> PISPIETVPVKLKPGMDGPKVKQWPLTEEKIKALVEICTEMEKEGKISKIGPENPYNTPVFAIKRKDSTKWRKLVDFRELNKRTQDFWEVQLGIPHPAGLKKKKSVTVLDVGDAYFSVPLDEDFRKYTAFTIPSINNETPGIRYQYNVLPQGWKGSPAIFQSSMTKILEPFKKQNPDIVIYQYMDDLYVGSDLEIGQHRTKIEELRQHLLRWGLTTPDKKHQKEPPFLWMGYELHPDKWTVQPIVLPEKDSWTVNDICKLVGKLNWASQIYPGIKVRQLSKLLRGTKALTEVIPLTEEAELELAENREILKEPVHGVYYDPSKDLIAEIQKQGQGQWTYQIYQEPFKNLKTGKYARMRGAHTNDVKQLTEAVQKITTESIVIWGKTPKFKLPIQKETWETWWTEY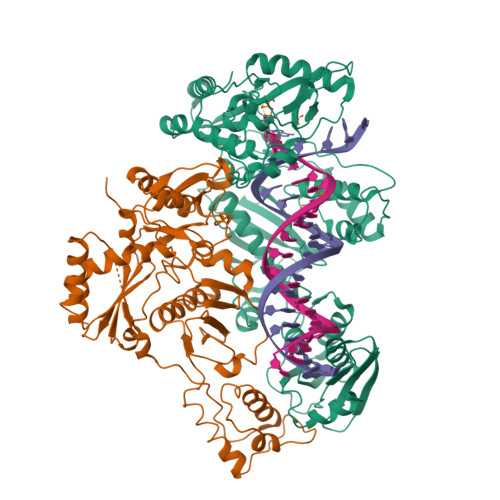WQATWIPEWEFVNTPPLVKLWYQLEKEPIVGAETFYVDGAANRETKLGKAGYVTNKGRQKVVPLTNTTNQKTELQAIYLALQDSGLEVNIVTDSQYALGIIQAQPDKSESELVNQIIEQLIKKEKVYLAWVPAHKGIGGNEQVDKLVSAGIRK;> PISPIETVPVKLKPGMDGPKVKQWPLTEEKIKALVEICTEMEKEGKISKIGPENPYNTPVFAIKKKDSTKWRKLVDFRELNKRTQDFWEVQLGIPHPAGLKKKKSVTVLDVGDAYFSVPLDEDFRKYTAFTIPSINNETPGIRYQYNVLPQGWKGSPAIFQSSMTKILEPFKKQNPDIVIYQYMDDLYVGSDLEIGQHRTKIEELRQHLLRWGLTTPDKKHQKEPPFLWMGYELHPDKWTVQPIVLPEKDSWTVNDIQKLVGKLNWASQIYPGIKVRQLSKLLRGTKALTEVIPLTEEAELELAENREILKEPVHGVYYDPSKDLIAEIQKQGQGQWTYQIYQEPFKNLKTGKYARMRGAHTNDVKQLTEAVQKITTESIVIWGKTPKFKLPIQKETWETWWTEYWQATWIPEWEFVNTPPLVKLWYQLGGHHHHHH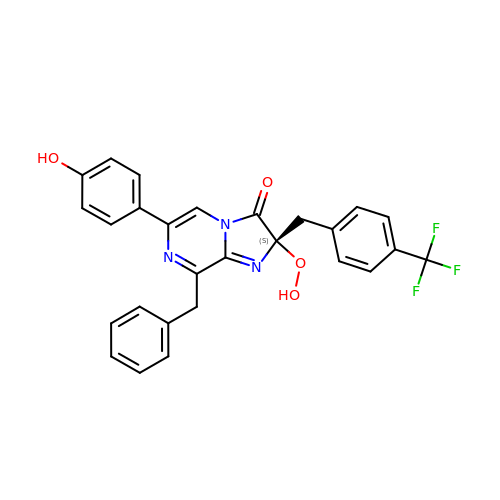(2S)-8-benzyl-2-hydroperoxy-6-(4-hydroxyphenyl)-2-{[4-(trifluoromethyl)phenyl]methyl}imidazo[1,2-a]pyrazin-3(2H)-one | C27 H20 F3 N3 O4 | ISIFAODRJRHDGD-SANMLTNESA-N>HHHHHHMSRLSEPSPYVEFDRRQWRALRMSTPLALTEEELVGLRGLGEQIDLLEVEEVYLPLARLIHLQVAARQRLFAATAEFLGEPQQNPDRPVPFIIGVAGSVAVGKSTTARVLQ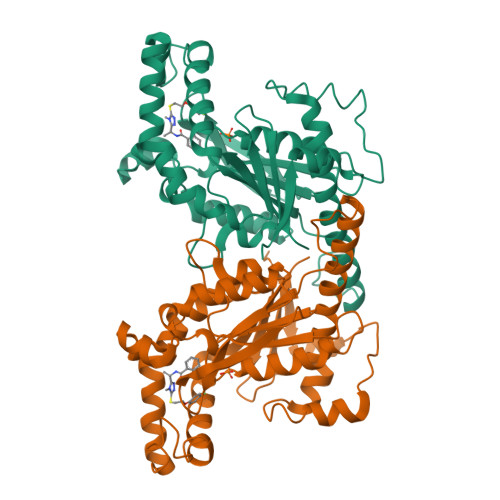ALLARWDHHPRVDLVTTDGFLYPNAELQRRNLMHRKGFPESYNRRALMRFVTSVKSGSDYACAPVYSHLHYDIIPGAEQVVRHPDILILEGLNVLQTGPTLMVSDLFDFSLYVDARIEDIEQWYVSRFLAMRTTAFADPESHFHHYAAFSDSQAVVAAREIWRTINRPNLVENILPTRPRATLVLRKDADHSINRLRLRKL[2x]>[4x]EKNVKEITDATKEPYNSVVAFVGGTGVVVGKNTIVTNKHIAKSNDIFKNRVSAHHSSKGKGGGNYDVK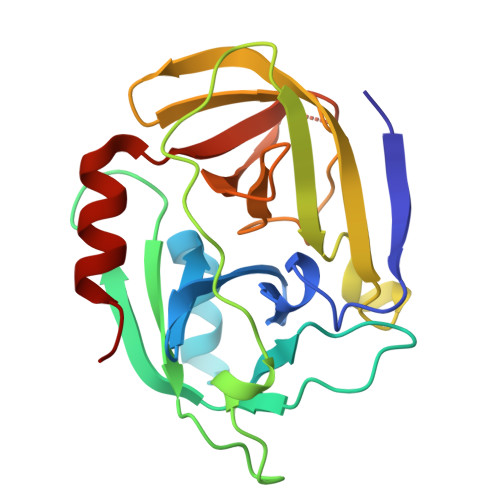DIVEYPGKEDLAIVHVHETSTEGLNFNKNVSYTKFADGAKVKDRISVIGYPKGAQTKYKMFESTGTINHISGTFMEFDAYAQPGNSGSPVLNSKHELIGILYAGSGKDESEKNFGVYFTPQLKEFIQNNIEK>[4x]MHHHHHHLKNGMRPIHPGEILREEFQKEMGFSAAALARALGVATPTVNNILRERGGVS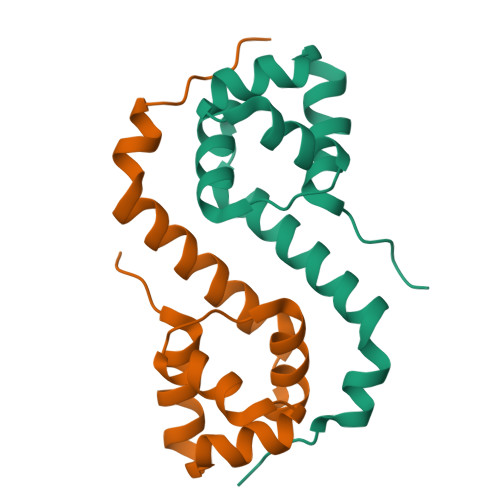ADMALRLSICLDTTPEFWLNLQTAFDLRTAEQQHGDEIIGSVQRLVA Contractile bacteriophages of the family Myoviridae (i.e. T4), R-type pyocins and the type VI secretion system (T6SS) of Gram-negative bacteria are evolutionarily related nano-scale injection machines that puncture target cell membranes using a shared contraction mechanism. TssA subunits are enigmatic as they possess a conserved N-terminal region of unknown function, previously identified as ImpA_N (PFAM: PF0681226), whereas sequences located C-terminal to this region are highly divergent. Consistent with this, phylogenetic analysis has suggested that the TssA family can be subdivided into three clades (TssA1, TssA2 and TssA3). The structural studies presented here show that TssA1B, TssA2A and TssA2B possess structurally diverse CTDs that lead to distinct overall architectures for their respective complexes.

Nested deletion of consecutive helical segments of TssA1B CTD revealed that loss of α15 resulted in the failure of the protein to assemble into a high molecular weight ring, and structure determination of the construct H12–H14 (helices α12–α14) and of that consisting of α12 and α13 alone (residues 303–347), revealed them both to be dimers. In the assembled Bc TssA1B CTD ring, analysis by PISA32 revealed an extensive dimer interface (~950 Å2) between monomers in the different layers, which principally involves the interaction of residues located in helices α12–α13 with their two-fold related subunits forming a region of hydrophobic packing with hydrophilic interactions at the periphery.

>ISHMIQNRAQAVDQLRAVARYFRQTEPHSPVAYLADKAAEWADMPLHKWLESVVKDDGSLSHIRELLGVRPDEQS[2x]> ALLDETPLPPGSRLDVRAYTTVLHALSRAGRYERALELFAELRRQGVAPTVVTYNTLIDGLCKAGKLDEALKLFEEMVEKGIKPDVVTYNTLIDGLCKAGKLDEALKLFEEMVEKGIKPDVVTYNTLIDGLCKAGKLDEALKLFEEMVEKGIKPDVVTYNTLIDGLCKAGKLDEALKLFEEMVEKGIKPDVVTYTTLIDGLCKAGKLDEALKLFEEMVEKGIKPDVVTYTTLI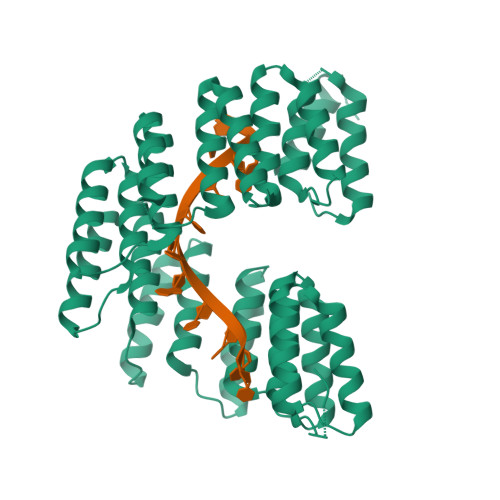DGLCKAGKLDEALKLFEEMVEKGIKPDVVTYNTLIDGLCKAGKLDEALKLFEEMVEKGIKPDVVTYNTLIDGLCKAGKLDEALKLFEEMVEKGIKPDVVTYNTLIDGLCKAGKLDEALKLFEEMVEKGIKPDVVTYNTLIDGLCKAGKLDEALKLFEEMVEKGIKPDELTYRRVVESYCRAKRFEEARGFLSEVSETDLDFDKKALEAYIEDAQFGRLEHHHHHHHH>[7x]TTTVGLVCKDGVVMATEKRATMGNFIASKAAKKIYQIADRMAMTTAGSVGDAQFLARIIKIE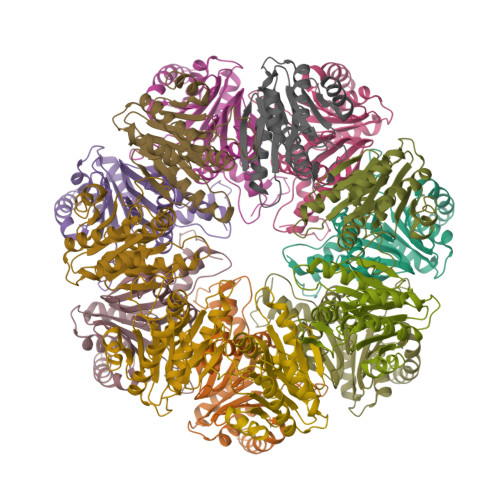ANLYEIRRERKPTVRAIATLTSNLLNSYRYFPYLVQLLIGGIDSEGKSIYSIDPIGGAIEEKDIVATGSGSLTAYGVLEDRFTPEIGVDEAVELAVRAIYSAMKRDSASGDGIDVVKITEDEFYQYSPEEVEQILAKFRK;>ITVFSPDGRLFQVEYAREAVKRGATAIGIKCKEGVILIADKRVGSKLLEADTIEKIYKIDEHICAATSGLVADARVLIDRARIEAQINRLTYDEPITVKELAKKICDFKQQYTQYGGVRPFGVSLLIAGVDEVPKLYETDPSGALLEYKATAIGMGRNAVTEFFEKEYRDDLSFDDAMVLGLVAMGLSIESELVPENIEVGYVKVDDRTFKEVSPEELKPYVERANERIRELLKK[7x]(5R)-5-[3-(4-fluorophenyl)-1-phenyl-1H-pyrazol-4-yl]imidazolidine-2,4-dione 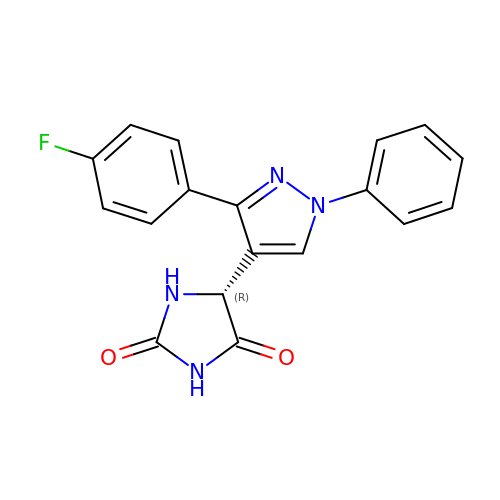| C18 H13 F N4 O2 | MPQWYPLPWGUMJE-MRXNPFEDSA-N>[6x]MARGLVIGEALIDIVDGPDPAEYVGGSPLNVAVGLARLGRDVDLLTHIGRDARGRRIAEYIESSGVQLVSGSQ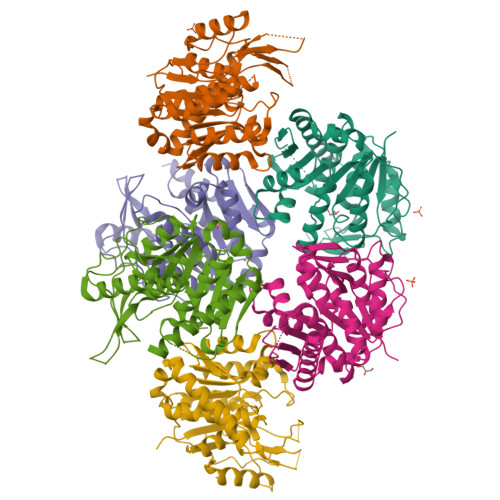TADRTPTATARIGPDGSATYAFDLEWQIPDTPPVAPPLLVHTGSIAAAREPGCLAVAALLDAYRAAATVSFDPNVRPSLSADPDLTRERIQRLVERSDIIKASAEDLHWIDPTQPPEQTARAWLACGPAIVALTLGDQGAVAFCAAGPASVPAQPVRVVDTVGAGDAFMAGLLDTLWEQGLLGADRRTELRKIGVSALTSALEVAALTSALTVARAGADLPYRADLRQSR Bacterial contractile injection systems (CIS) are phage tail-like macromolecular complexes that mediate cell-cell interactions by injecting effector proteins into target cells. Using Streptomyces coelicolor as a model organism, we and others previously demonstrated that S. coelicolor CIS (CISSc) mediate a form of regulated cell death, which influences the onset of sporulation and secondary metabolite production in response to exogenous stress and unknown cellular signals (Casu et al., 2023; Vladimirov et al., 2023). The purified assemblies were subjected to single-particle cryo-electron microscopy (cryoEM) for structure determination, yielding the first high-resolution model of the CISSc in its extended conformation, which also presents the first example of a CIS IId subtype. Our model shows that extended CISSc particles share the conserved eCIS architecture, including the three core modules: cap, sheath tube, and baseplate.

The distal end of the CISSc is capped by a tail terminator complex. This cap comprises one protein, Cis16, forming a C6-symmetrical complex that terminates the inner tube and sheath, respectively. (e) Top view (left) and side view (right) of ribbon diagrams showing the cap module of CISSc, revealing that the cap is composed of a Cis16 hexamer. The resulting maps of the baseplate and the cap reached resolutions of 3.5 and 3.4 Å, respectively.

>MIHEVDEVLKALLKGGALTDSGIDVAFEAPTRDWAARRNAPVVNAYLYDIREDVGRRHRGQVAVRDQDDIVVKRRQPPRWFRLSYLVTAWTKTPQDEHRLLSAVLATLLPREQLPPYELPGALGAMNLPVPMTVAGVQTESRSLAEIWSALGGELKPSLDLVVTAPFPAYPEYDAGPPVTEGATVRIGGVEGDPPMSEGRSHRPHQVAAARAARKAVTDGRTKRQ[6x];>[6x]MSLPKPEDVLVAPNFGIQIDGVMVEYLNSVSNLQIEQDVIRYQQNQGTTGRNNVTLMPGVAKDGSVQVERGMSQSSVFTQWINDSMAGRMATARKNATIIVMDYEDNPVKRWNLRNAWCSKVVAGTLKAGDTNALTETITIVFEELVVE;>MPSYLSPGVYVEEVASGSRPIEGVGIEGVGTSVAAFVGLAPTGPLNEPTLVTNWTQYVAAFGDFTGGYYLAHSVYGFFNNGGSAAYVVRVGGSAEDAAADGSVNGAAAPAAVTGSTAKALPAAEPKQLGTFAVTATAAGQSGPLTVEVADPEGEGPAERFKLIVKDGDKPVETFDVSAKKGNRSYVVTQVKERSKLITVTEAAPSAQLVRPENQSLTLPAPPSAAPAVPAGQAESAHPGPAQYLGDSSDRTGFGGLEAIDEISMVAVPDLMAAYQRGAIDLEAVKAVQLGLIAHCELMGDRVAIIDPPPNQNARQIRVWRQETAGYDSKYAALYYPWIKSFDPATGQSRLVPPSGHVAGIWARNDSERGVHKAPANEVVRGAVDLELQITRGEQDLLNPIGVNCIRSFPGRGIRVWGARTLSSDPAWRYLNIRRYFNYLEESILIGTQWVVFEPNDHNLWARIRRNVSAFLVNEWRNGALFGQSPDQAYYVKCDEETNPPESVDLGRVVCEIGIAPVKPAEFVIFRLAQFSSGGGELDE[6x]> LPENVDWRKKGAVTPVRHQGSCGSCWAFSAVATVEGINKIRTGKLVELSEQELVDCERRSHGCKGGYPPYALEYVA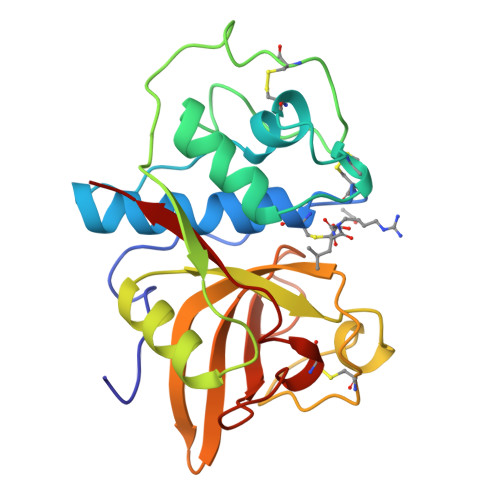KNGIHLRSKYPYKAKQGTCRAKQVGGPIVKTSGVGRVQPNNEGNLLNAIAKQPVSVVVESKGRPFQLYKGGIFEGPCGTKVEHAVTAVGYGKSGGKGYILIKNSWGTAWGEKGYIRIKRAPGNSPGVCGLYKSSYYPTKN>[4x]MKKLFLVFWWHMHQPLYREPYTGEYLLPWTFFHAVKDYYDMPAYLKDFEIKLNFNLTPVLIDQIQEYAQGKAKDVFLEAIRKDPDDLEKEEVEKLIEFTKLNYEKPIYRFERIRELMNKEKLNREELLDLQTLNLLAWCGRTLRKDLKDLLNKGRNYTQEEKEYVLNKYFEIIKKTLSIYREIKEEGKGSVSTSP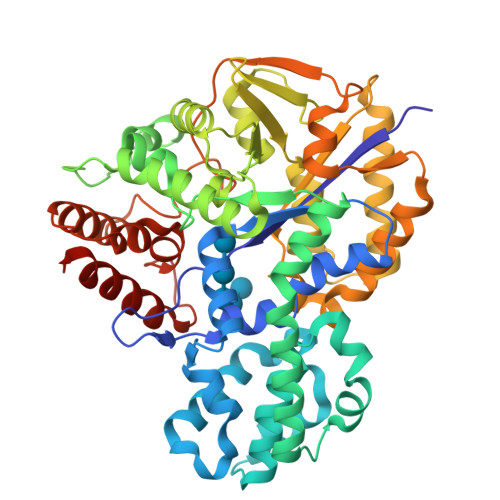YYHPLIPILLNPNCVYETTPNVKIPDFAVSFREDASKHVELAKEKYFEIFGEHPVYMWPPQASVSNEALELYYEKGINMLATDEVILKNSVERASPYLRYYFRELISVFFRDKTLSDLIGFSYHAWNAEDAVRDFIGRLKKIHESVDFQPVVFVVLDGENCWEYYEENGIPFLEKLYSTLEKEEWIETLTLEEAMRKEDVKTEVIESVKAGTWFDGNFLKWIGNKEKNEYWKILIEAKKKAKNDYILVAEGSDWFWWQGEEKAPFVEVFDKLFRSFVRRAQELEHHHHHH> AGRLEEALELFEEMKEKGIVPDVVTYNTLISGLGKAGRLEEALELFEEMKEKGIVPDVVTYTTLISGLGKAGRLEEALELFEEMKEKGIVPNVVTYTTLISGLGKAGRLEEALELFEEMKEKGIVPDVVTYTTLISGLGKAGRLEEALELFEEMKEKGIVPDVVTYTTLISGLGKAGRLEEALELFEEMKEKGIVPDVVTYNTLISGLGKAGRLEEALELFEEMKEKGIVPDVVTYNTLISGLGKAGRLEEALELFEEMKEKGIV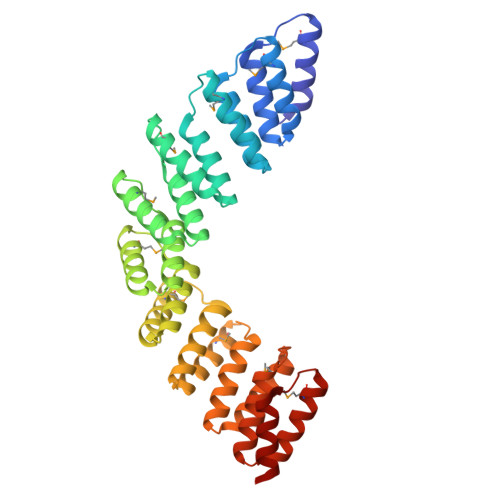PDVVTYTTLISGLGKAGRLEEALELFEEMKEKGIVPNVVTYTTLISGLGKAGRLEEALELFEEMKEKGIVPDVVTYTTLISGLGK> MPADSSSNNTKNTIDIPPTTVKGRDNYDFYGRVDIESNPTDLNATNLTRYNYGQPPGTTTAGAVQFKNQVSFDKDFDFNIRVANNRQSNTTGADGWGFMFSKKDGDDFLKNGGILREKGTPSAAGFRIDTGYYNNDPLDKIQKQAGQGYRGYGTFVKNDSQGNTSKVGSGTPSTD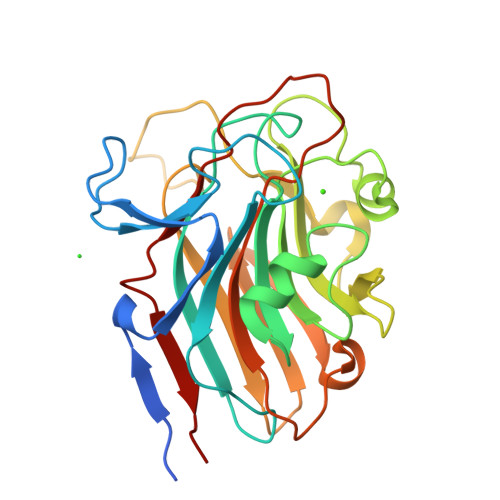FLNYADNTTNDLDGKFHGQKLNNVNLKYNASNQTFTATYAGKTWTATLSELGLSPTDSYNFLVTSSQYGNGNSGTYASGVMRADLDGATLTYTPKA> GSGGSGKVVKFSYMWTINNFSFCREEMGEVIKSSTFSSGANDKLKWCLRVNPKGLDEESKDYLSLYLLLVSCPKSEVRAKFKFSILNAKGEETKAMESQRAYRFVQGKDWGFKKFIRRGFLLDEANGLLPDDKLT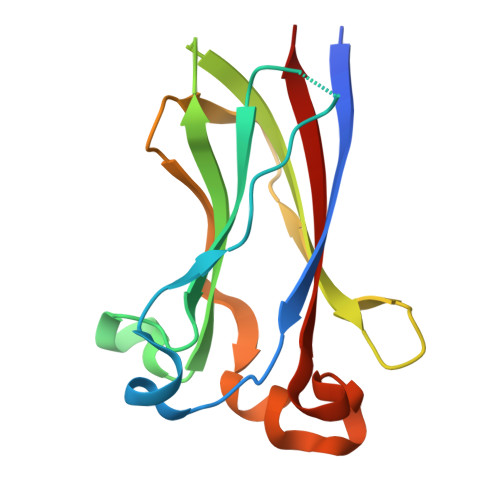LFCEVSVVQD(2R,3R)-4-(4-AMINO-1H-IMIDAZO[4,5-C]PYRIDIN-1-YL)-2,3-DIHYDROXYBUTANOIC ACID | C10 H12 N4 O4 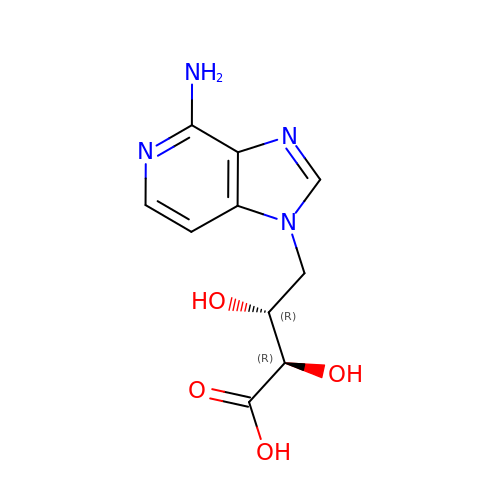| PBWCZGPIALILAS-HTRCEHHLSA-N N,N'-(1H-PYRROLE-2,5-DIYLDI-4,1-PHENYLENE)DIBENZENECARBOXIMIDAMIDE | C30 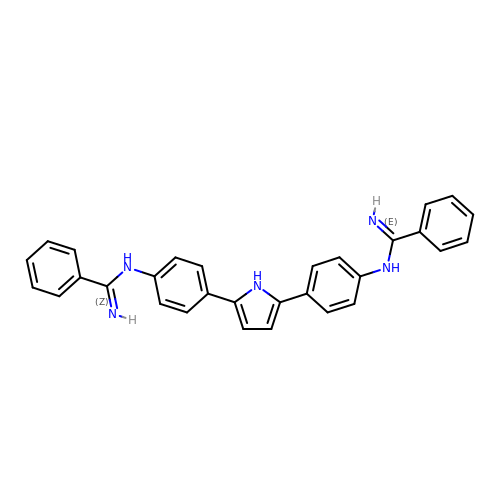H25 N5 | AXUZUHYCWFMCLV-UHFFFAOYSA-N> GGGAACCCAUGCUUCAGUCAG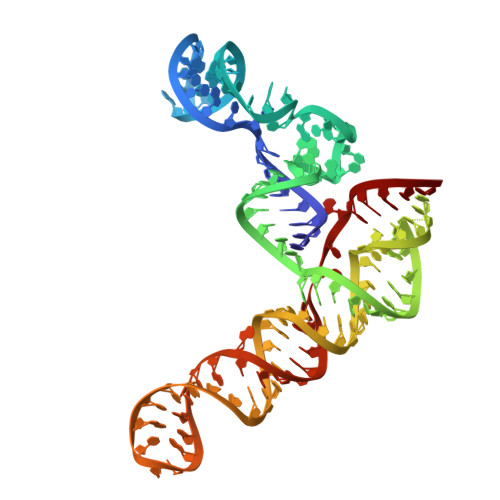CUGAUGCACAAUCGUUUUUAAACGGGUUUCCGGUGUAAGUGCAGCCCGUCUUACACCGUGCGGCACAGGCACUAGUACUGAUGUCGUAUACAGGGCU> SDWPNHARSPGN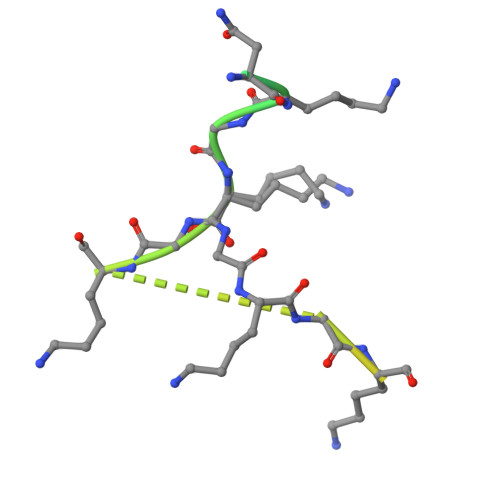KGKGKGKGKGKPKSQACEPSE> GPLSRKGIIPEEYVLTRLAEDPAEPRYRTRERRVDGSGSGSGSAAGSGSGSGSGSGAAAEDLQDLGVRFLQPFVNLLSKGTYWWMNAFIKTAHKKPIDLRAIGKLPIAMRALTNYQRLCVAFDAQARKDTQSPQGARAIWRALCHAFGRRLILSSTFRILADLLGFAGPLCIFGIVDHLGKENHVFQPKTQFLGVYFVSSQEFLGNAYVLAVLLFLALLLQRTFLQASYYVAIETGINLRGAIQTKIYNKIMHLSTSNLSMGEMTAGQICNLVAIDTNQLMWFFFLCPNLWAMPVQIIVGVILLYYILGVSALIGAAVIILLAPVQYFVATKLSQAQRSTLEHSNERLKQTNEMLRGMKLLKLYAWESIFCSRVEVTRRKEMTSLRAFAVYTSISIFMNTAIPIAAVLITFVGHVSFFKESDLSPSVAFASLSLFHILVTPLFLLSSVVRSTVKALVSVQKLSEFLSSAEIREEQCAPREPAPQGQAGKYQAVPLKVVNRKRPAREEVRDLLGPLQRLAPSMDGDADNFCVQIIGGFFTWTPDGIPTLSNITIRIPRGQLTMIVGQVGCGKSSLLLATLGEMQKVSGAVFWNSNLPDSEGEDPSSPERETAAGSDIRSRGPVAYASQKPWLLNATVEENITFESPFNKQRYKMVIEACSLQPDIDILPHGDQTQIGERGINLSGGQRQRISVARALYQQTNVVFLDDPFSALDVHLSDHLMQAGILELLRDDKRTVVLVTHKLQYLPHADWIIAMKDGTIQREGTLKDFQRSECQLFEHWKTLMNRQDQELEKETVMERKASEPSQGLPRAMSSRDGLLLDEEEEEEEAAESEEDDNLSSVLHQRAKIPWRACTKYLSSAGILLLSLLVFSQLLKHMVLVAIDYWLAKWTDSALVLSPAARNCSLSQECDLDQSVYAMVFTLLCSLGIVLCLVTSVTVEWTGLKVAKRLHRSLLNRIILAPMRFFETTPLGSILNRFSSDCNTIDQHIPSTLECLSRSTLLCVSALTVISYVTPVFLVALLPLAVVCYFIQKYFRVASRDLQQLDDTTQLPLLSHFAETVEGLTTIRAFRYEARFQQKLLEYTDSNNIASLFLTAANRWLEVRMEYIGACVVLIAAATSISNSLHRELSAGLVGLGLTYALMVSNYLNWMVRNLADMEIQLGAVKRIHALLKTEAESYEGLLAPSLIPKNWPDQGKIQIQNLSVRYDSSLKPVLKHVNALISPGQKIGICGRTGSGKSSFSLAFFRMVDMFEGRIIIDGIDIAKLPLHTLRSRLSIILQDPVLFSGTIRFNLDPEKKCSDSTLWEALEIAQLKLVVKALPGGLDAIITEGGENFSQGQRQLFCLARAFVRKTSIFIMDEATASIDMATENILQKVVMTAFADRTVVTIAHRVHTILSADLVMVLKRGAILEFDKPETLLSQKDSVFASFVRADK

The KATP channel is a hetero-octamer complex composed of four pore-forming Kir6 (kir6.1 or Kir6.2) subunits and four regulatory sulfonylureas receptor subunits (SUR1 or SUR2). KATP channels can sense intracellular ATP/ADP ratio using the inhibitory ATP binding site on Kir6 and the activating Mg–ADP binding site on SUR, coupling the metabolism status of the cell to its membrane potential. In pancreatic β-cells, KATP channels are mainly formed by Kir6.2 and SUR1, and play key roles in controlling insulin secretion. Small-molecule drugs that inhibit the pancreatic KATP channel are widely used to boost insulin secretion for the treatment of diabetes and are therefore named insulin secretagogues (ISs).

Therefore, we used a truncated construct (SUR1core) that encompasses 208-1582 of SUR1, including TMD1, NBD1, TMD2, and NBD2, for subsequent structure determination. Purified SUR1core protein was supplemented with ATP and MTG for cryo-EM sample preparation and data collection. Image processing yielded a reconstruction with an overall resolution of 3.27 Å. In the presence of ATP and MTG, SUR1core shows an inward-facing conformation with its central vestibule widely open to the cytosol. ATP binds to the NBD1 and MTG binds inside a pocket in the central vestibule of SUR1. The MTG-binding pocket is formed by residues on TM7 and TM8 of TMD1 and TM16 and TM17 of TMD2. The central negatively charged carboxyl group of MTG makes electrostatic interactions with positively charged R1246 on TM16 and R1300 on TM17. The benzene ring of MTG stacks with the phenyl group of F433. The bulky hexahydro-2-isoindoline group binds in a hydrophobic pocket surrounded by L1241 and T1242 of TMD2 and I381, I385, F433, and W430 of TMD1. In agreement with this, the hexahydro-2-isoindoline group of MTG is near the S1238, and the replacement of S1238 with a tyrosine would generate sterical clashes with MTG, abolishing its binding.> MEHVAFGSEDIENTLAKMDDGQLDGLAFGAIQLDGDGNILQYNAAEGDITGRDPKQVIGKNFFKDVAPC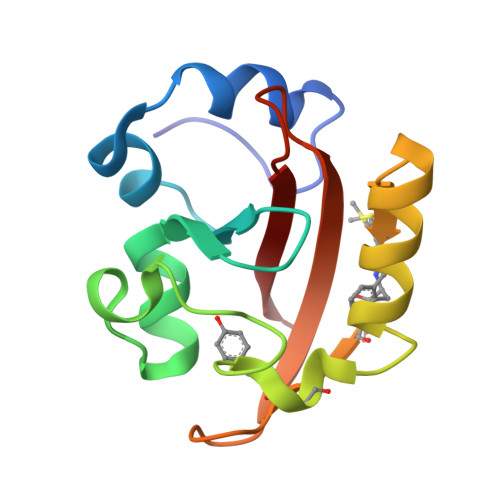TDSPEFYGKFKEGVASGNLNTMXEYTFDYQMTPTKVKVHMKKALSGDSYWVFVKRV> AHMQEAANRSPPYAPYPYPVDEIIGGDSVQSIQRRLLGTNWNPSAHDMQMSRIQAEDLFELKVEI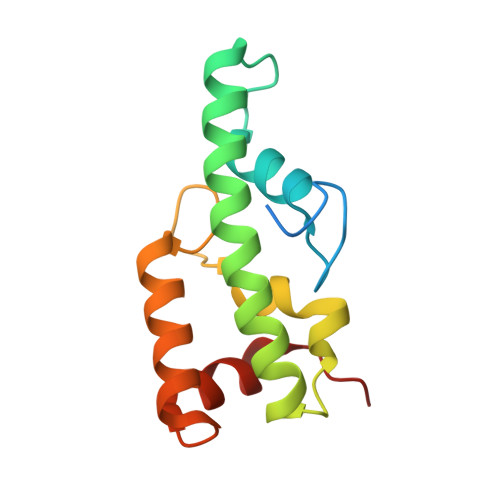IRKMAGLHPSGDWMGWGARALDNPRTATGEEDLARLHQMLDDLQSRNEQSATFWRLVERVRLRAD Anti‐CRISPR (Acr) proteins, which are naturally occurring inhibitors of CRISPR‐Cas systems, have evolved as a counterdefense mechanism employed by bacteriophages and other mobile genetic elements. The AcrVIA6 protein, which targets the type VI‐A CRISPR‐Cas system, has been identified as a potent Cas13a inhibitor. While an initial study suggested that AcrIVA6 is a true anti‐CRISPR protein, another study argued that AcrIVA6 might not be an anti‐CRISPR due to its inability to inhibit Cas13 activity in an in vivo system. However, there is currently conflicting debate regarding the anti‐CRISPR function of AcrVIA6. This study reveals that AcrVIA6 functions as a DNA‐binding protein rather than a Cas13a inhibitor, as it does not block RNA cleavage.

The protein was crystallized, and its structure was solved at 2.39 Å. The high‐resolution structure of AcrVIA6 revealed a five‐helical bundle fold, modeled from residues 4–85. The helices (α1–α5) span residues 12–25, 29–36, 40–48, 54–67, and 69–85. Electrostatic analysis showed predominantly positive charges. Finally, we analyzed the amino acid conservation using the Consurf server to infer functionally important residues in AcrVIA6. This analysis revealed that Q9, P10, and G11, belonging to the N‐terminal loop, as well as F72, Y76, and R79 in the last helix α5, are completely conserved, along with several conserved glycine residues in the middle. The top five hits, including the transcription regulator C.Esp1396I, were all DNA‐binding proteins. Hence, AcrVIA6 exists as a monomer in a solution, unlike other structurally similar DNA‐binding proteins that form dimers. The long N‐terminal loop, impeding dimer formation, is a distinctive feature of AcrVIA6 and contributes to its binding to dsDNA as a monomer. Therefore, AcrVIA6 is a dsDNA‐binding protein that uses the HTH motif, comprising α2 and α3, to bind dsDNA. Using an in vitro Cas13a activity assay, we confirmed that AcrVIA6 fails to inhibit RNA cleavage, even at high concentrations.

> MADKVKSIQPGPIFYDVFLVYLRVIGTNLKDWCAPHGVTATNAKSAATGGWNGTKARALRQKMIDEVGEETFLRLYTERLRREAALEHHHHHH> MSRGSMEGQGCCGGGGGKTEMIPTEEALRIVFGVSKRLPPVIVSLYEALGKVLAEDIRAPDPLPPYPASVKDGYAVVASDGPGEYPVITESRAGNDGLGVTVTPGTVAYVTTGGPIPDGADAVVQVEDTKVIGDVSTESKRVKILIQTKKGTDIRRVGCDIEKDATVLTTGERIGASEIGLLATAGVTMVKVYPMPIVAILSTGDELVEPTAGTLGRGQIRDSNRAMLVAAVMQQQCKVVDLGIVRDDRKELEKVLDEAVSSGVDIILTSGGVSMGDRDFVKPLLEEKGKVYFSKVLMAPGKPLTFAEIRAKPTESMLGKTVLAFGLPGNPVSCLVCFNIFVVPTIRQLAGWTSPHPLRVRLRLQEPIKSDPIRPEFHRAIIKWKDNDGSGTPGFVAESTGHQMSSRLLSMRSANALLELPATGNVLSAGSS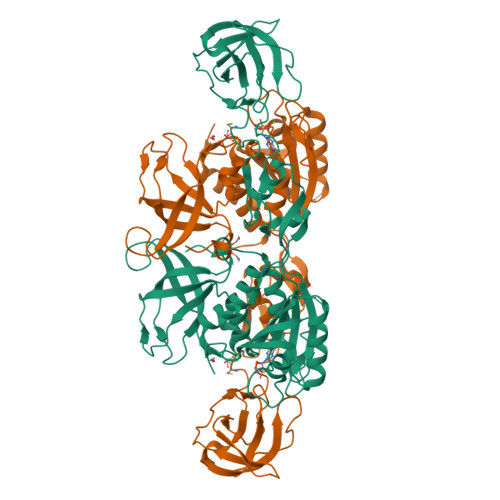VSAIIVSDISAFSIDKKASLSEPGSTSGGSAWSHPQFEK>[2x]MNLLVTSSLGVLLHLVVLCQADDHSELLVNTKSGKVMGTRVPVLSSHISAFLGIPFAEPPVGNMRFRRPEPKKPWSGVWNASTYPNNCQQYVDEQFPGFSGSEMWNPNREMSEDCLYLNIWVPSPRPKSTTVMVWIYGGGFYSGSSTLDVYNGKYLAYTEEVVLVSLSYRVGAFGFLALHGSQEAPGNVGLLDQRMALQWVHDNIQFFGGDPKTVTIFGESAGGASVGMHILSPGSRDLFRRAILQSGSPNCPWASVSVAEGRRRAVELGRNLNCNLNSDEELIHCLREKKPQELIDVEWNVLPFDSIFRFSFVPVIDGEFFPTSLESMLNSGNFKKTQILLGVNKDEGSFFLLYGAPGFSKDSESKISREDFMSGVKLSVPHANDLGLDAVTLQYTDWMDDNNGIKNRDGLDDI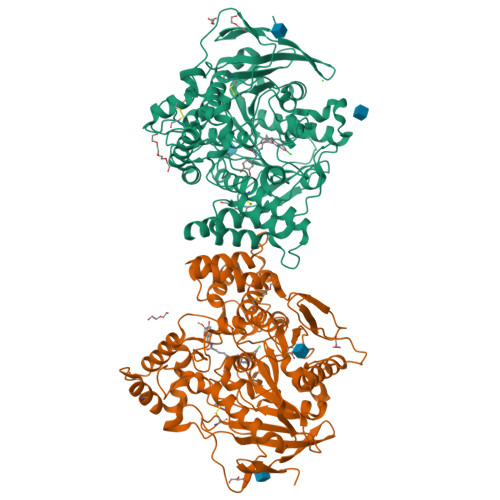VGDHNVICPLMHFVNKYTKFGNGTYLYFFNHRASNLVWPEWMGVIHGYEIEFVFGLPLVKELNYTAEEEALSRRIMHYWATFAKTGNPNEPHSQESKWPLFTTKEQKFIDLNTEPMKVHQRLRVQMCVFWNQFLPKLLNATACDGELSSSGTSSSKGIIFYVLFSILYLIF Apolipoprotein B messenger RNA-editing enzyme, catalytic polypeptide-like (APOBEC3) proteins are single-stranded DNA (ssDNA) deoxycytidine deaminases that are among some of the fastest evolving proteins in the human genome. APOBEC3s catalyse a cytidine (C) to uridine (U) zinc-dependent deamination reaction. APOBEC3A (A3A) is a single-domain enzyme with the highest catalytic activity among the human APOBEC3 proteins. All APOBEC3 domains contain a HAEx28Cx2-4C zinc binding motif.

The crystal structure of A3A (E72A/C171A) in complex with ssDNA was determined by molecular replacement at 2.2 Å resolution. E72A inactivates the enzyme permitting the formation of stable complexes and C171A increases solubility. A 15-mer DNA oligonucleotide that binds A3A with ∼60 nM affinity26 with a target deoxycytidine (5′-TTTTTTTCTTTTTTT-3′) was co-crystallized with A3A. The target deoxycytidine (dC0) and flanking deoxythymidines (dT−1 and dT1), as well as one additional deoxyribose at 5′-end and one phosphate at 3′-end, were well ordered in the electron density (5′-sugar-dT−1-dC0-dT1-phosphate-3′). The central cytidine (dC0) and the preceding thymidine (dT−1) are accommodated in a deep groove formed by Loops 1,3,5 and 7 of A3A. The bound DNA adopts an irregular conformation to encircle the side chain of H29. Compared to apo A3A, there are conformational changes in the rotamers of the side chains of R28 and H29 in Loop 1, and Y132 in Loop 7, accompanied by more subtle reorganization of N57–A72 in loop 3. The deoxycytidine (dC0), which is the target of deamination reaction, is well coordinated and buried within the active site of A3A. As expected for a catalytic A3 domain, electron density that fits a zinc ion was observed coordinating H70, C101, C106 as well as additional density that fits a Cl− ion, with both assignments confirmed by anomalous difference calculations. The structure explains this strong conservation, as N57 of A3A is central in recognizing ssDNA with three key distinct interactions: The side chain of N57 determines the 5′–3′ directionality of ssDNA binding by forming a hydrogen bond to O3′ atom of dC0, which helps stabilize the geometry of the DNA backbone and the sugar in a C2′-endo conformation and induces a backbone deformation due to steric hindrance with O5′ of the target dC0.

> GPGHMEASPASGPRHLMDPHIFTSNFNNGIGRHKTYLCYEVERLDNGTSVKMDQHRGFLHNQAKNLLCGFYGRHAALRFLDLVPSLQLDPAQIYRVTWFISWSPCFSWGCAGEVRAFLQENTHVRLRIFAARIYDYDPLYKEALQMLRDAGAQVSIMTYDEFKHCWDTFVDHQGAPFQPWDGLDEHSQALSGRLRAILQNQGN> SLGP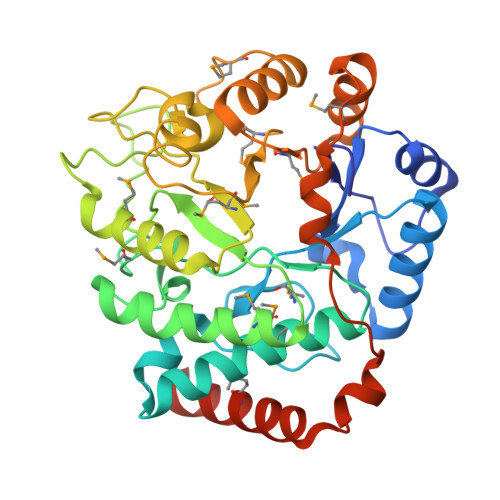LWLDVAGYELSAEDREILQHPTVGGVILFGRNYHDNQQLLALNKAIRQAAKRPILIGVDQEGGRVQRFREGFSRIPPAQYYARAENGVELAEQGGWLMAAELIAHDVDLSFAPVLDMGFACKAIGNRAFGEDVQTVLKHSSAFLRGMKAVGMATTGKHFPGHGAVIADSHLETPYDERETIAQDMAIFRAQIEAGVLDAMMPAHVVYPHYDAQPASGSSYWLKQVLREELGFKGIVFSDDLSMEGAAVMGGPVERSHQALVAGCDMILICNKREAAVEVLDNLPIMEVPQAEALLKKQQFSYSELKRLERWQQASANMQRLIEQFSEEGGSHHHHHH N-(2,3-dichlorophenyl)-4-[(isoquinolin-5-yl)sulfonyl]piperazine-1-carboxamide 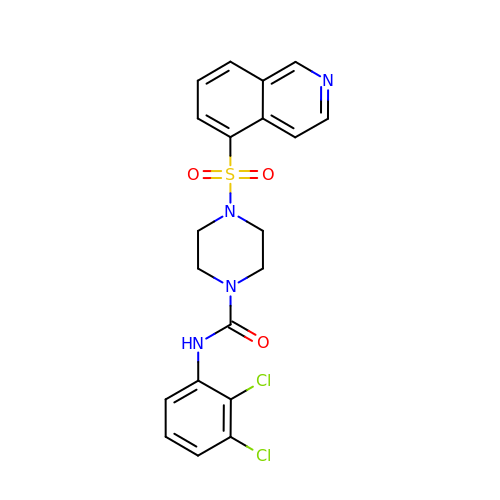| C20 H18 Cl2 N4 O3 S | OPIJBEYHDBKGKX-UHFFFAOYSA-N>SVLFPCKYASSGCEITLPHTEKADHEELCEFRPYSCPCPGASCKWQGSLDAVMPHLMHQHKSITTLQGEDIVFLATDINLPGAVDWVMMQSCFGFHFMLVLEKQEKYDGHQQFFAIVQLIGTRKQAENFAYRLELNGHRRRLTWEATPRSIHEGIATA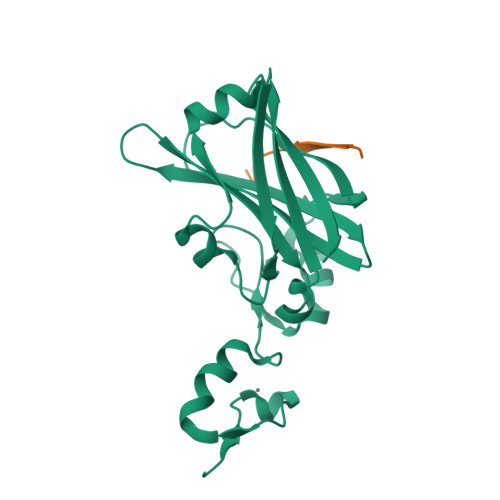IMNSDCLVFDTSIAQLFAENGNLGINVTISMC[4x];>[4x]YRVPKEVRVEPQKFAEELIH>[3x]MAAPMTPAARPEDYEAALNAALADVPELARLLEIDPYLKPYAVDFQRRYKQFSQILKNIGENEGGIDKFSRGYESFGVHRCADGGLYCKEWAPGAEGVFLTGDFNGWNPFSYPYK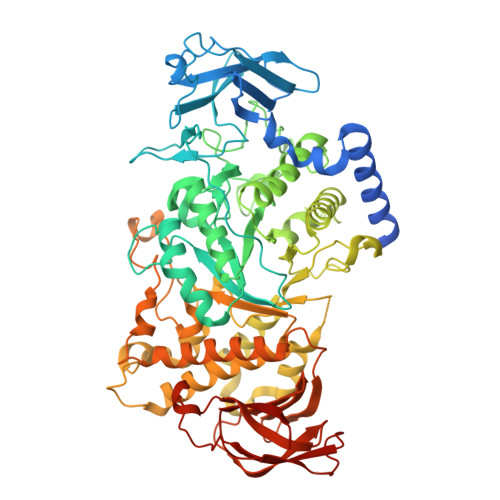KLDYGKWELYIPPKQNKSVLVPHGSKLKVVITSKSGEILYRISPWAKYVVREGDNVNYDWIHWDPEHSYEFKHSRPKKPRSLRIYESHVGISSHEGKVASYKHFTCNVLPRIKGLGYNCIQLMAIMEHAYYASFGYQITSFFAASSRYGSPEELQELVDTAHSMGIIVLLDVVHSHASKNSADGLNMFDGTDSCYFHSGPRGTHDLWDSRLFAYSSWEVLRFLLSNIRWWLEEYRFDGFRFDGVTSMLYHHHGVGQGFSGDYSEYFGLQVDEDALTYLMLANHLVHTLCPDSITIAEDVSGMPALCSPISQGGGGFDYRLAMAIPDKWIQLLKEFKDEDWNMGDIVYTLTNRRYLEKCIAYAESHDQALVGDKSLAFWLMDAEMYTNMSVLTPFTPVIDRGIQLHKMIRLITHGLGGEGYLNFMGNEFGHPEWLDFPRKGNNESYHYARRQFHLTDDDLLRYKFLNNFDRDMNRLEERYGWLAAPQAYVSEKHEGNKIIAFERAGLLFIFNFHPSKSYTDYRVGTALPGKFKIVLDSDAAEYGGHQRLDHSTDFFSEAFEHNGRPYSLLVYIPSRVALILQNVDLPN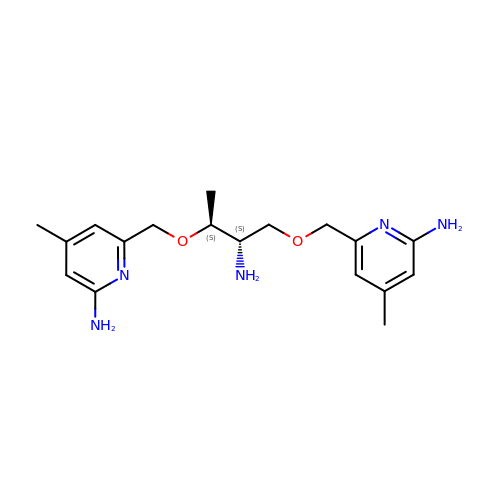6,6'-{[(2S,3S)-2-aminobutane-1,3-diyl]bis(oxymethanediyl)}bis(4-methylpyridin-2-amine) | C18 H27 N5 O2 | BGQWILAWEWZMTG-BBRMVZONSA-N>[2x]MPTSNPAKPLDGFRVLDFTQNVAGPLAGQVLVDLGAEVIKVEAPGGEAARQITSVLPGRPPLATYFLPNNRGKKSVTVDLTTEQAKQQMLRLADTADVVLEAFRPGTMEKLGLGPDDLRSRNPNLIYARLTAYGGNGPHGSRPGIDLVVAAEAGMTTGMPTPEGKPQII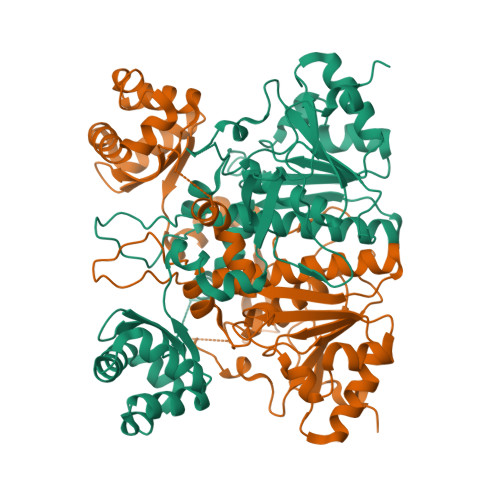PFQLVANASGHVLAQAVLAALLHRERNGVADVVQVAMYDVAVGLQANQLMMHLNRAASDQPKPEPAPKAKRRKGVGFATQPSDAFRTADGYIVISAYVPKHWQKLCYLIGRPDLVEDQRFAEQRSRSINYAELTAELELALASKTATEWVQLLQANGLMACLAHTWKQVVDTPLFAENDLTLEVGRGADTITVIRTPARYASFRAVVTDPPPTAGEHNAVFLARP> PGASVPTEETCKSCVCTNSSQVVCRPEEGKILNQTQDGAFCYWEICGPNGTVEKHFNICSITTRPSTLTTFTTITLPTTPTSFTTTTTTTTPTSSTVLSTTPKLCCLWSDWINEDHPSSGSDDGDRETFDGVCGAPEDIECRSVKDPHLSLEQHGQKVQCDVSV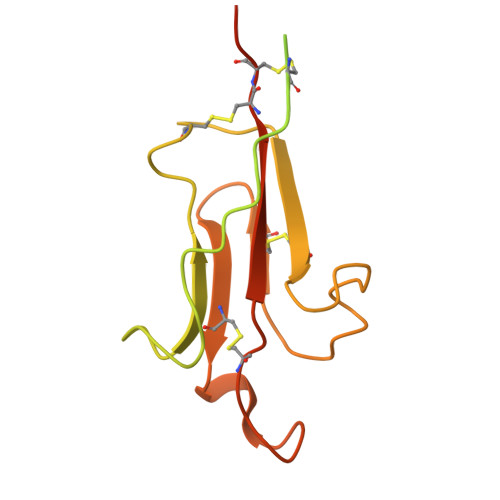GFICKNEDQFGNGPFGLCYDYKIRVNCCWPMDKCITHHHHHH Protein tyrosine phosphatases (PTPs) play a critical role in regulating cellular functions by selectively dephosphorylating their substrates. The ∼280 residue PTP catalytic domain consists of an α/β structure, and biochemical and structural studies have led to a detailed understanding of the catalytic mechanism (Barford et al., 1994; Zhang, 2002). Key features of the domain include the PTP signature motif, the mobile Trp-Pro-Asp “WPD” loop that in the closed conformation positions the conserved and catalytically important aspartate residue, and the phosphotyrosine recognition loop. Here we report the crystal structures of 22 PTP domains, including two tandem-domain RPTP structures and a detailed structural comparison of this protein family.

In the fourth category, both the gateway and secondary pocket are blocked and the inaccessible binding cavity harbors an aromatic residue or a proline in position of Arg24. The second-site loop assumes a twisted conformation in these phosphatases. This architecture is present in the subgroups NT5 (PTPH1, MEG1), NT6 (PTPD1, PTPD2), R1 (CD45), R2B (RPTPμ, RPTPκ, RPTPρ), and R4 (RPTPα, RPTPɛ). PTPs with particularly high enzymatic activity against generic substrates were RPTPσ and PTP subgroups R5, R3, NT1, NT2, NT3, NT4, and NT5. The subgroups NT1, NT2, NT3, and NT5 exhibited a pronounced preference for acidic residues N-terminal to the phosphorylation site.

> SMEEKLENEPDFQYIPEKAPLDSVHQDDHSLRESMIQLAEGLITGTVLTQFDQLYRKKPGMTMSCAKLPQNISKNRYRDISPYDATRVILKGNEDYINANYINMEIPSSSIINQYIACQGPLPHTCTDFWQMTWEQGSSMVVMLTTQVERGRVKCHQYWPEPTGSSSYGCYQVTCHSEEGNTAYIFRKMTLFNQEKNESRPLTQIQYIAWPDHGVPDDSSDFLDFVCHVRNKRAGKEEPVVVHCSAGIGRTGVLITMETAMCLIECNQPVYPLDIVRTMRDQRAMMIQTPSQYRFVCEAILKVYEEGFVKPLTTSTNKLT> MLNQELELSLNMAFARAREHRHEFMTVEHLLLALLSNPSAREALEACSVDLVALRQELEAFIEQTTPVLPASEEERDTQPTLSFQRVLQRAVFHVQSSGRNEVTGANVLVAIFSEQESQAAYLLRKHEVSRLDVVNFISHGTRKDEPTQSSDPGSQPNSEEQAGGEERLENFTTNLNQLARVGGIDPLIGREKELERAIQVLCRRRKNNPLLVGESGVGKTAIAEGLAWRIVQGDVPEVMADCTIYSLDIGSLLAGTKYRGDFEKRFKALLKQLEQDTNSILFIDEIHTIIGAGAASGGQVDAANLIKPLLSSGKIRVIGSTTYQEFSNIFEKDRALARRFQ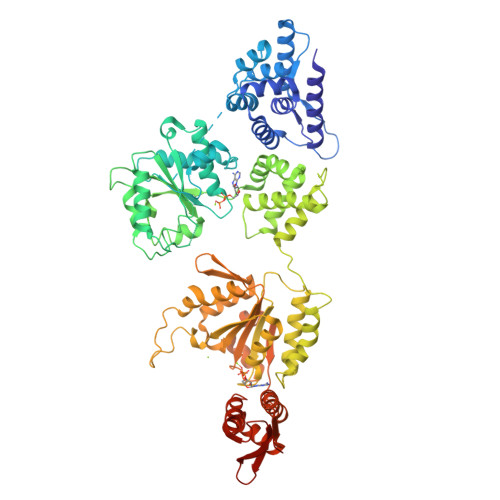KIDITEPSIEETVQIINGLKPKYEAHHDVRYTAKAVRAAVELAVKYINDRHLPDKAIDVIDEAGARARLMPVSKRKKTVNVADIESVVARIARIPEKSVSQSDRDTLKNLGDRLKMLVFGQDKAIEALTEAIKMARAGLGHEHKPVGSFLFAGPTGVGKTEVTVQLSKALGIELLRFDMSEYMERHTVSRLIGAPPGYVGFDQGGLLTDAVIKHPHAVLLLDEIEKAHPDVFNILLQVMDNGTLTDNNGRKADFRNVVLVMTTNAGVRETERKSIGLIHQDNSTDAMEEIKKIFTPEFRNRLDNIIWFDHLSTDVIHQVVDKFIVELQVQLDQKGVSLEVSQEARNWLAEKGYDRAMGARPMARVIQDNLKKPLANELLFGSLVDGGQVTVALDKEKNELTYGFQSAQKHKAEAAH> SVVGRFRLIVPAATAKPSPAIGQTLGPLGINMMQFCKEFNARTANVRPEVPLQVTIVPLTDRSYKFSIRAPSNIWFLLRTARCPMGSE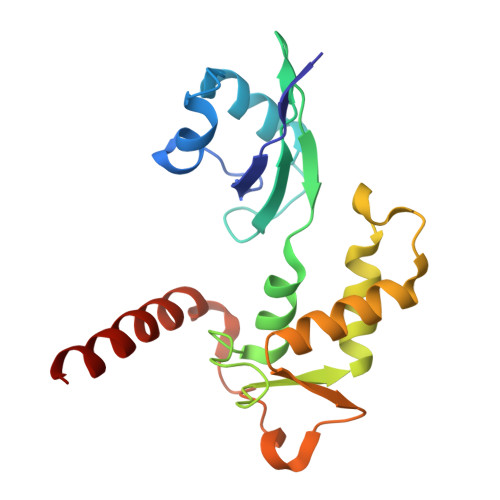SPGHQSVGNVTLKEIYHIARCKSMDWPLIGMSLRGICRSLIGTARASGIEISKEILPAYHKRDYTDVQALDSMRKDMRQRKKAAKRAAT> MGSSHHHHHHSQDPMSLNLVSEQLLAANGLKHQDLFAILGQLAERRLDYGDLYFQSSYHESWVLEDRIIKDGSYNIDQGVGVRAISGEKTGFAYADQISLLALEQSAQAARTIVRDSGDGKVQTLGAVEHSPLYTSVDPLQSMSREEKLDILRRVDKVAREADKRVQEVTASLSGVYELILVAATDGTLAADVRPLVRLSVSVLVEEDGKRERGASGGGGRFGYEFFLADLDGEVRADAWAKEAVRMALVNLSAVAAPAGTMPVVLGAGWPGVLLHAAVGHGLEGDFNRRGTSVFSGQVGELVASELCTVVDDGTMVDRRGSVAIDDEGTPGQYNVLIENGILKGYMQDKLNARLMGMTPTGNGRRESYAHLPMPRMTNTYMLPGKSTPQEIIESVEYGIYAPNFGGGQVDITSDKFVFSTSEAYLIENGKVTKP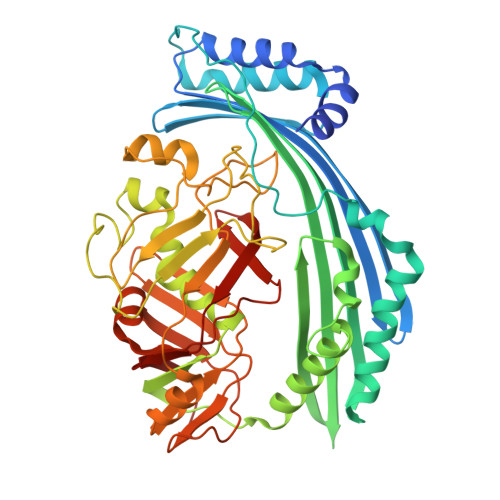VKGATLIGSGIETMQQISMVGNDLKLDNGVGVCGKEGQSLPVGVGQPTLKVDNLTVGGTA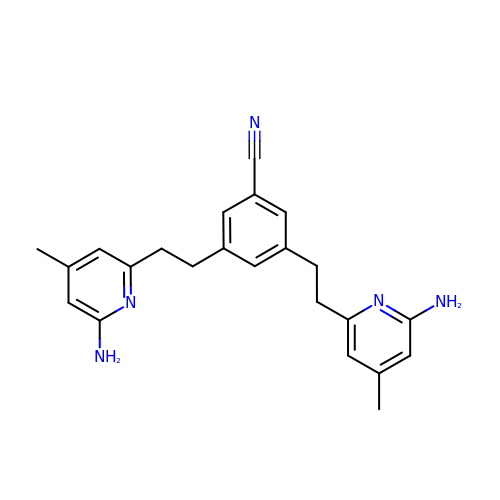3,5-bis[2-(6-amino-4-methylpyridin-2-yl)ethyl]benzonitrile | C23 H25 N5 | IXUSJKAERUMZME-UHFFFAOYSA-N>[6x]LVPRGSHMAKKVRFYRNGDRYFKGIVYAVSSDRFRSFDALLADLTRSLSDNIN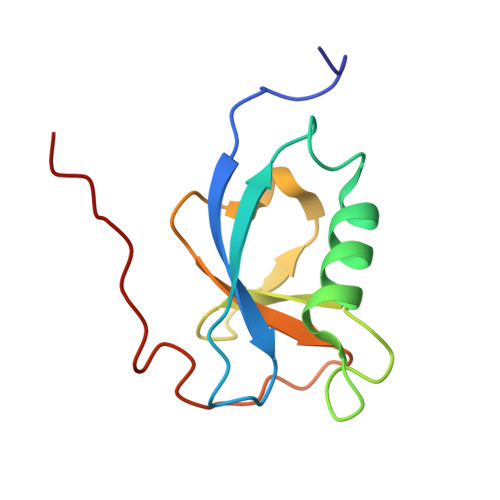LPQGVRYIYTIDGSRKIGSMDELEEGESYVCSSDNFFDDVEYTKNVNPNWSVNV1,2-HYDRO-1-OXY-3,4-HYDRO-3-(1-METHOXY-2-OXY-3,4-DIHYDROXYPENTYL)-8,9-DIHYROXY-7-METHYLANTHRACENE 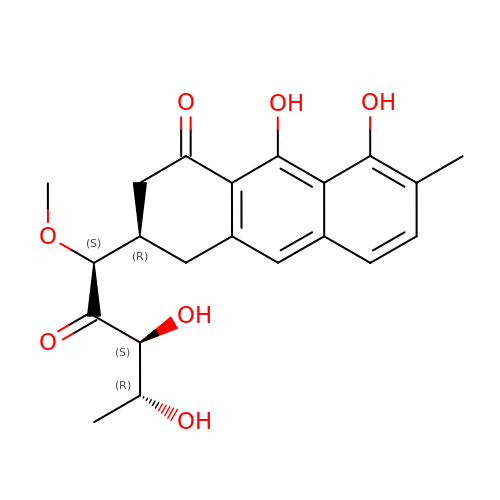| C21 H24 O7 | XBKVKSRQTHGEJA-FAGSEQTRSA-N> LDFNYHRQEGMEAFLKTVAQNYSSV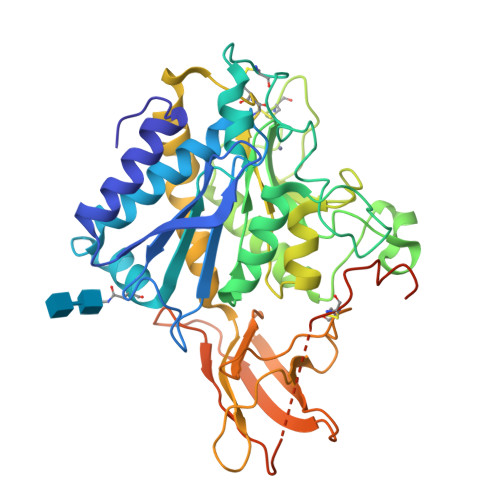THLHSIGKSVKGRNLWVLVVGRFPKEHRIGIPEFKYVANMHGDETVGRELLLHLIDYLVTSDGKDPEITNLINSTRIHIMPSMNPDGFEAVKKPDCYYSIGRENYNQYDLNRNFPDAFEYNNVSRQPETVAVMKWLKTETFVLSANLHGGALVASYPFDNGVQATGALYSRSLTPDDDVFQYLAHTYASRNPNMKKGDECKNKMNFPNGVTNGYSWYPLQGGMQDYNYIWAQCFEITLELSCCKYPREEKLPSFWNNNKASLIEYIKQVHLGVKGQVFDQNGNPLPNVIVEVQDRKHICPYRTNKYGEYYLLLLPGSYIINVTVPGHDPHITKVIIPEKSQNFSALKKDILLPFQGQLDSIPVSNPSCPMIPLYRNLPDHSAATKPSLFLFLVSLLHIFFK2-[3-[(4-azanyl-2-methyl-pyrimidin-5-yl)methyl]-4-methyl-2H-1,3-thiazol-5-yl]ethyl phosphono hydrogen phosphate | C12 H20 N4 O7 P2 S | 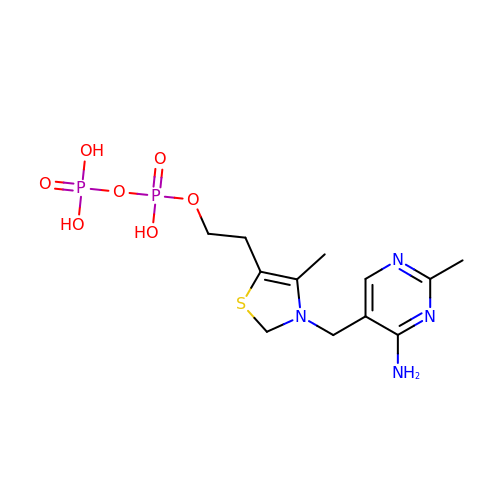FCUXBJDJFWOWMD-UHFFFAOYSA-N>[2x]MSMIETWTAVDQYVSDVLIPKDSTLEEVLQVNAAANLPAHDVSPTQGKFLQLLVQIQGARNILEIGTLGGYSTIWLARGLSSGGRV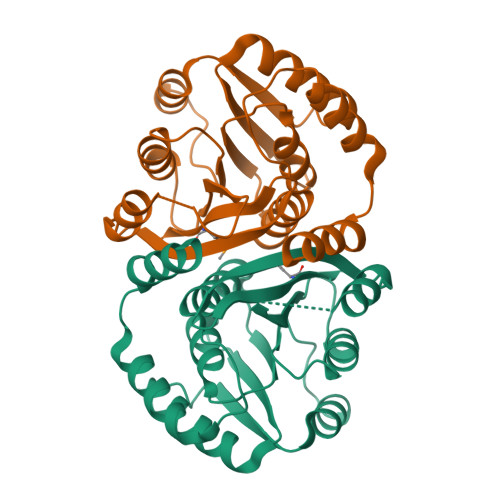VTLEASEKHADIARSNIERANLNDRVEVRTGLALDSLQQIENEKYEPFDFIFIDADKQNNPAYFEWALKLSRPGTVIIGDNVVREGEVIDNTSNDPRVQGIRRFYELIAAEPRVSATALQTVGSKGYDGFIMAVVKE> 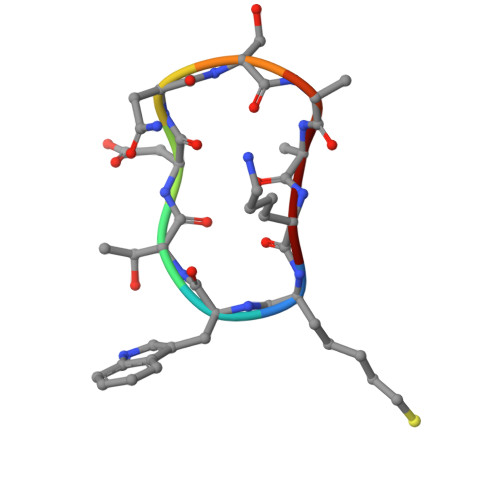XWTDNSMDK>GSSGSSGMQIGKIIKVSGPLVMAENMSEASIQDMCLVGDLGVIGEIIEMRQDVASIQVYEETSGIGPGEPVRSTGEALSVELGPGIISQMFDGIQRPLDTFMEVTQSNFLGRGVQLPALDHEKQWWFEATIEEGTEVSAGDIIGYVDETKIIQHKIMVPNGIKGTVQKIESGSFTIDDPICVIETEQGLKELTMMQKWPVRRGRPIKQKLNPDVPMITGQRVIDTFFPVTKGGAAAVPGPFGAGKTVVQHQIAKWSDVDLVVYVGCGERGNEMTDVVNEFPELIDPNTGESLMERTVLIANTSNMPVAAREASIYTGITIAEYFRDMGYDVAIMADSTSRWAEALREMSGRLEEMPGDEGYPAYLGSRLAEYYERSGRVIALGSDQREGSITAISAVSPSGGDISEPVTQNTLRVVKVFWGLDSSLAQKRHFPSINWIQSYSLYSTEVGRYMDQILQQDWSDMVTEGMRILQEEEQLNEIVRLVGIDSLSDNDRLTLEVAKSIREDYLQQNAFDDVDTFTSREKQFNMLKVILTFGKEARKALSLGAYFNEIMEGTVAVRERISRSKYIPEEELAKISSINEEIKETIQLIVSEGGMTDD[3x];>[3x]GSSGSSGMIKEYRTIKEVVGPLMAVEKVSGVKYEELIEVRMQNGEIRRGQVLEVQEDKAMVQIFEGTSGINYKNSSVRFLGHPLQLGVSEDMIGRVFDGLGRPKDNGPEILPEKYLDINGEVINPIARDYPDEFIQTGISAIDHLNTLVRGQKLPVFSGSGLPHKELAAQIARQATVLDSSDDFAVVFAAIGITFEEAEFFMEDFRQTGAIDRSVMFMNLANDPAIERIATPRMALTAAEYLAYEKGMHVLVIMTDMTNYAEALREISAARREVPGRRGYPGYLYTNLATLFERAGRIRGLKGSVTQIPILTMPEDDKTHPIP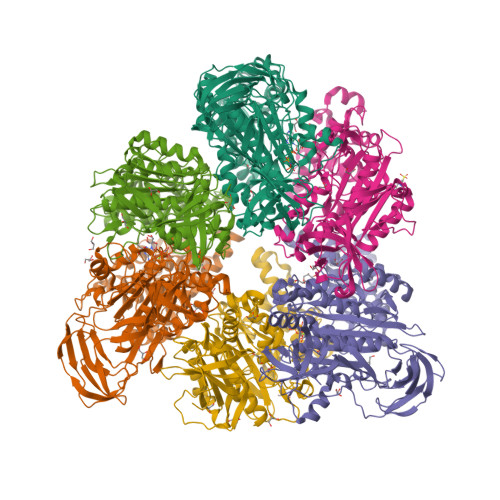DLTGYITEGQIILTRELYKSGIQPPIDVLPSLSRLKDKGTGAGKTREDHAATMNQLFAAYAQGKQAKELAVVLGESALSDIDKIYAKFAERFENEYVNQGFYTNRTITETLDLGWELLAMLPRTELKRIKDDLLDKYLPEGK> MSAIPITPTKRIRRNLFDDAPATPPRPLKRKKLQFTDVTPESSPEKLQFGSQSIFLRTKALLQKSSELVNLNSSDGALPARTAEYEQVMNFLAKAISEHRSDSLYITGPPGTGKTAQLDMIIRQKFQSLPLSLSTPRSKDVLRHTNPNLQNLSWFELPDGRLESVAVTSINCISLGEPSSIFQKIFDSFQDLNGPTLQIKNMQHLQKFLEPYHKKTTFVVVLDEMDRLLHANTSETQSVRTILELFLLAKLPTVSFVLIGMANSLDMKDRFLSRLNLDRGLLPQTIVFQPYTAEQMYEIVIQKMSSLPTIIFQPMAIKFAAKKCAGNTGDLRKLFDVLRGSIEIYELEKRFLLSPTRGSLNSAQVPLTPTTSPVKKSYPEPQGKIGLNYIAKVFSKFVNNNSTRTRIAKLNIQQKLILCTIIQSLKLNSDA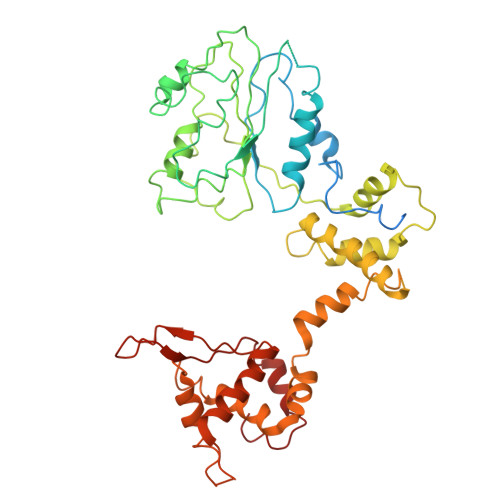TIDESFDHYIKAITKTDTLAPLQRNEFLEICTILETCGLVSIKKTKCKGKTKRFVDKIDVDLDMREFYDEMTKISILKPFLH NICOTINAMIDE PURIN-6-OL-DINUCLEOTIDE | C21 H26 N6 O15 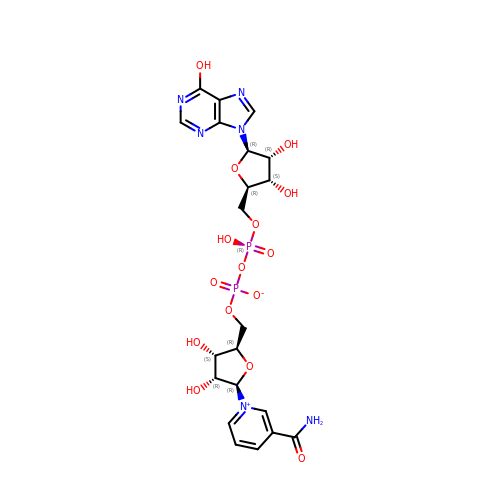P2 | DGVSIBCCYUVRNA-NNYOXOHSSA-N>[2x]GPLGSMIVFVRFNSSYGFPVEVDSDTSIFQLKEVVAKRQGVPADQLRVIFAGKELQNHLTVQNCDLEQQSIVHIVQRPQRKSHETNASGGSEAARGPAAKPTYHSFFVYCKGPCHKVQPGKLRVQCGTCRQATLTLAQGPSCWDDVLIPNRMSGECQSPDCPGTRAEFFFKCGAHPTSDKDTSVALNLITNNSRSIPCIACTDVRNPVLVFQCNHRHVICLDCFHLYCVTRLNDRQFVHDAQLGYSLPCVAGCPNSLIKELHHFRILGEEQYNRYQQYGAEECVLQMGGVLCPRPGCGAGLLPEQGQRKVTCEGGNGLGCGFVFCRDCKEAYHEGECDSMFEASGATSQAYRVDQRAAEQARWEEASKETIKKTTKPCPRCNVPIEKNGGCMHMKCPQPQCKLEWCWNCGCEWNRACMGDHWFDV

Parkin is a cytosolic E3 ubiquitin ligase that is recruited to mitochondria damaged by depolarization, reactive oxygen species (ROS), or accumulation of unfolded proteins (Narendra et al, 2008; Jin & Youle, 2013; Ashrafi et al, 2014). Parkin is a member of the RBR (RING-in-between-RING) ligase family, which uses a RING/HECT hybrid mechanism to transfer ubiquitin from an E2 enzyme to a substrate via a thioester intermediate (Wenzel et al, 2011). Parkin consists of an N-terminal Ubl domain, followed by a long linker leading to four zinc-binding domains: RING0, RING1, IBR, and RING2, collectively referred to as the R0RBR module. Crystal structures of full-length Parkin (Trempe et al, 2013) and the C-terminal domains (Riley et al, 2013; Trempe et al, 2013; Wauer & Komander, 2013) showed that under basal conditions, the protein adopts a closed conformation where multiple intramolecular interactions inhibit key sites that are required for ubiquitin transfer.

The length of this linker varies significantly between different species, so we designed a version lacking its least conserved section spanning residues 86–130 (Δ86–130 Parkin; Fig1A). This version of Parkin was crystallized and its structure was determined at a resolution of 2.54 Å (Fig1B). The higher resolution Δ86–130 Parkin structure superimposes well on the full-length Parkin structure (backbone rmsd of 1.6 Å), showing that the reduced length of the linker does not perturb the conformation of Parkin (FigEV1D). Intramolecular interactions between RING0 and RING2 block Cys431 in the catalytic site, and the E2-binding site is occluded by the Ubl domain and linker between the IBR and RING2 domains (Fig1B). The Ubl domain mainly interacts with helix 261–274 of the RING1 domain (Fig1E). Arg6 and His68 form hydrogen bonds with Asp274, a residue located at the end of the helix and preceding Arg275, a frequent mutation site in familial PD (R275W). Like ubiquitin, Ubl has a hydrophobic patch centered on Ile44, which stacks against Leu266 of RING1 helix 261–274 (Fig1E). Asn8, a residue conserved in Parkin orthologs, binds RING1 helix 309–316 via a hydrogen bond with Gln311 and Arg314 (Fig1F). The first and best-ordered site is on RING1 opposite the Ubl-binding surface and formed by Arg305 and Tyr312 (Fig1C). Ser65 of the Ubl domain, which is phosphorylated by PINK1 (Shiba-Fukushima et al, 2012; Kazlauskaite et al, 2014a), faces the disordered residues 382–391 preceding the REP helix and is located within only 12 Å from RING1 (Fig1B).> GSSST;> GLGQMLESMIDNTVRETVGAATSRDALPNTEASGPTHSKEIPALTAVETGATNPLVPSDTVQTRHVVQHRSRSESSIESFFARGACVTIMTVDNSASTTNKDKLFAVWKITYKDTVQLRRKLEFFTYSRFDMELTFVVTANFTETNNGHALNQVYQIMYVPPGAPVPEKWDDYTWQTSSNPSIFYTYGTAPARISVPYVGISNAYSHFYDGFSKVPLKDQSAALGDSLYGAASLNDFGILAVRVVNDHNPTKVTSKIRVYLKPKHIRVWCPRPPRAVAYYGPGVDYKDGTLTPLSTKDLTTY;> SPNIEACGYSDRVLQLTLGNSTITTQEAANSVVAYGRWPEYLRDSEANPVDQPTEPDVAACRFYTLDTVSWTKESRGWWWKLPDALRDMGLFGQNMYYHYLGRSGYTVHVQCNASKFHQGALGVFAVPEMCLAGDSNTTTMYTSYQNANPGEKGGTFTGTFTPDNNQTSPARRFCPVDYLLGNGTLLGNAFVFPHQIINLRTNNCATLVLPYVNSLSIDSMVKHNNWGIAILPLAPLNFASESSPEIPITLTIAPMCCEFNGLRNITLPRLQ;> GLPVMNTPGSNQYLTADNFQSPCALPEFDVTPPIDIPGEVKNMMELAEIDTMIPFDLSATKKNTMEMYRVRLSDKPHTDDPILCLSLSPASDPRLSHTMLGEILNYYTHWAGSLKFTFLFCGSMMATGKLLVSYAPPGADPPKKRKEAML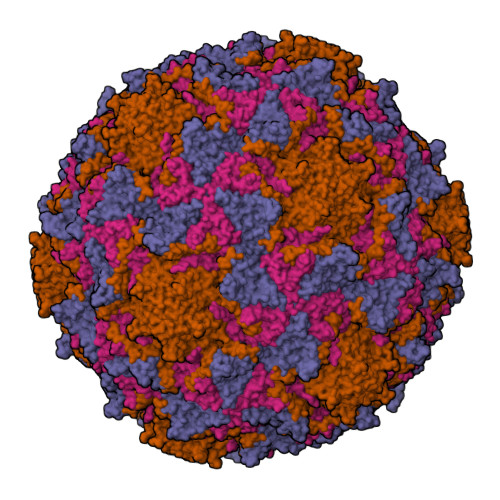GTHVIWDIGLQSSCTMVVPWISNTTYRQTIDDSFTEGGYISVFYQTRIVVPLSTPREMDILGFVSACNDFSVRLLRDTTHIEQKALAQ;> GAQVSSQKVGAHENSNRAYGGSTINYTTINYYRDSASNAASKQDFSQDPSKFTEPIKDVLIKTAPMLN>AAESGVSRPVPQLKRTTMRILIGLLVQNPELATLVPPLENLDENKLPGLGLFRELVNTCLSQPGLTTGQLLEHYRGTNNAATLEKLSMWDDIADKNIAEQTFTDS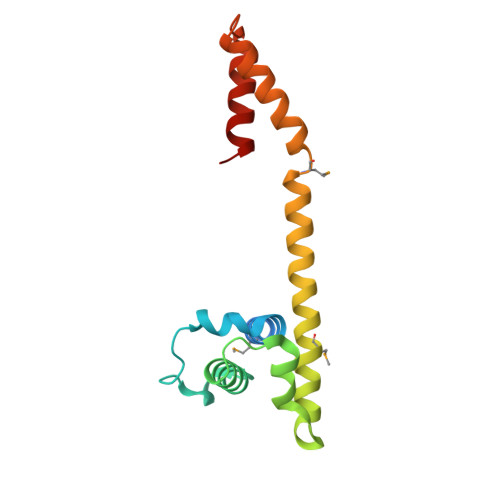LNHMFDSLLELRQEELIARERTHGLSNEERLELWTLNQELAKK[2x]> EIKTNSVEPIRHTYGHIARRFGDKPATRYQEASYDIEAKTNFHYRPQWDSEHTLNDPTRTAIRMEDWCAVSDPRQFYYGAYVGNRAKMQESAETSFGFCEKRNLLTRLSEETQKQLLRLLVPLRHVELGANMNNAKIAGDATATTVS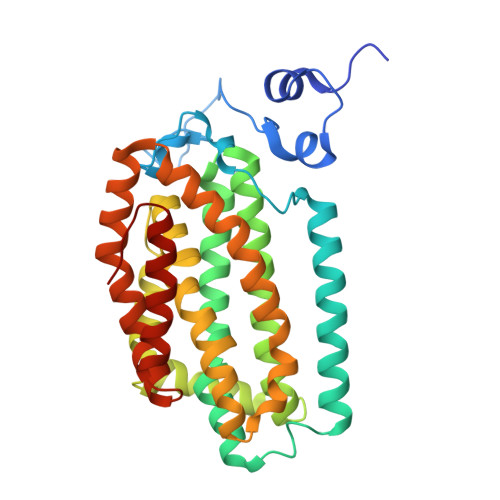QMHIYTGMDRLGIGQYLSRIALMIDGSTGAALDESKAYWMDDEMWQPMRKLVEDTLVVDDWFELTLVQNILIDGMMYPLVYDKMDQWFESQGAEDVSMLTEFMRDWYKESLRWTNAMMKAVAGESETNRELLQKWIDHWEPQAYEALKPLAEASVGIDGLNEARAELSARLKKFELQSRGV> RFQYLVKNQNLHIDYLAKKLHDIEEEYNKLTHDVDKKTIRQLKARISNLEEHHCDEHESECRGDVPECIHDLLFCDGEKDCRDGSDE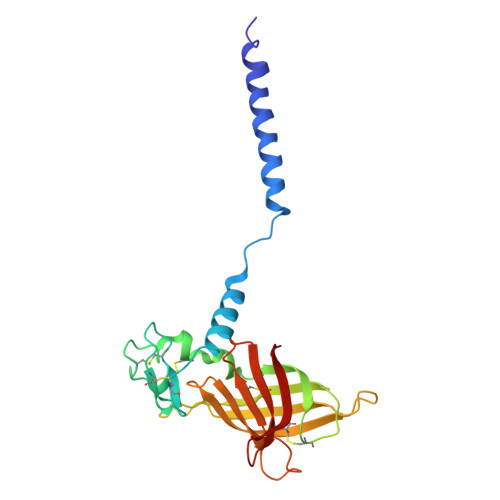DPETCSLNITHVGSSYTGLATWTSCEDLNPDHAIVTITAAHRKSFFPNRVWLRATLSYELDEHDHTVSTTQLRGFYNFGKRELLLAPLKGQSEGYGVICDFNLGDDDHADCKIVVPSSLFVCAHFNAQRY> GAPATVTEQGEDITSKKDRGVLKIVKRVGNGEETPMIGDKVYVHYKGKLSNGKKFDSSHDRNEPFVFSLGKGQVIKAWDIGVATMKKGEIAHLLIKP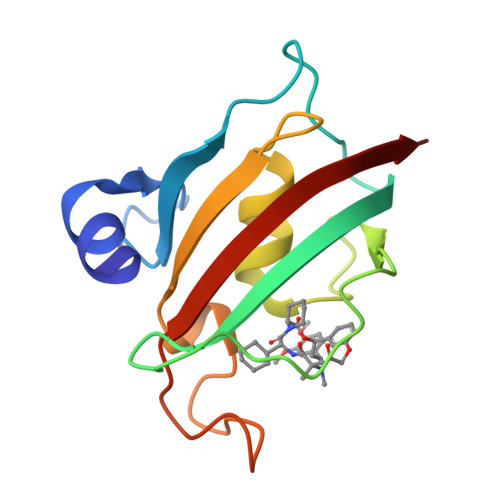EYAYGSAGSLPKIPSNATLFFEIELLDFKGE>[4x]GPLGSSEQQVAQDTEEVFRSYVFYLHQQEQETQGAAAPANPEMDNLPLEPNSILG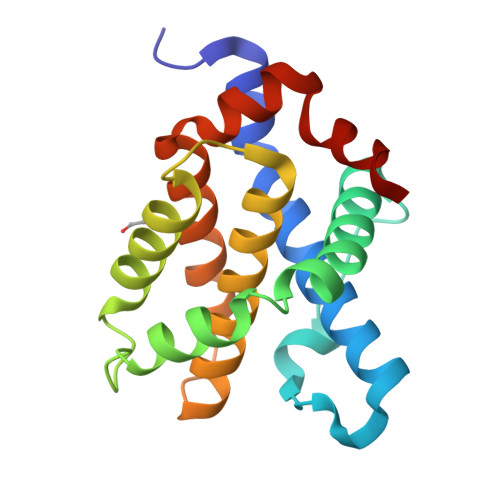QVGRQLALIGDDINRRYDTEFQNLLEQLQPTAGNAYELFTKIASSLFKSGISWGRVVALLGFGYRLALYVYQRGLTGFLGQVTSFLADIILHHYIARWIAQRGGWVAALNFRRD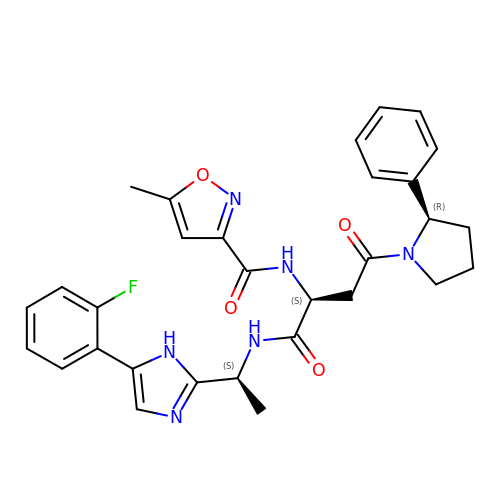N-{(2S)-1-({(1S)-1-[5-(2-fluorophenyl)-1H-imidazol-2-yl]ethyl}amino)-1,4-dioxo-4-[(2R)-2-phenylpyrrolidin-1-yl]butan-2-yl}-5-methyl-1,2-oxazole-3-carboxamide | C30 H31 F N6 O4 | KYSUEPWILKTYPX-FPDDQMOCSA-N>LTAKHRPSVVWLHNAECTGCTEAAIRTIKPYIDALILDTISLDYQETIMAAAGEAAEAALHQALEGKDGYYLVVEGGLPTIDGGQWGMVAGHPMIETTKKAAAKAKGIICIGTCSAYGGVQKAKPNPSQAKGVSEALGVKTINIPGCPPNPINFVGAVVHVLTKGIPDLDENGRPKLFYGELVHDNCPRLPHFEASEFAPSFDSEEAKKGFCLYELGCKGP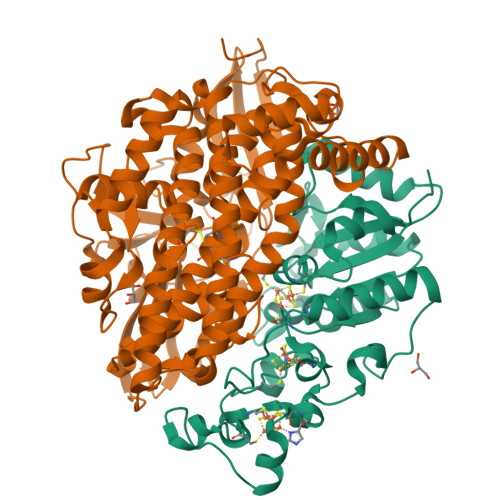VTYNNCPKVLFNQVNWPVQAGHPCLGCSEPDFWDTMTPFYEQG[3x];>[3x]MAESKPTPQSTFTGPIVVDPITRIEGHLRIMVEVENGKVKDAWSSSQLFRGLEIILKGRDPRDAQHFTQRACGICTYVHALASSRCVDDAVKVSIPANARMMRNLVMASQYLHDHLVHFYHFHALDWVDVTAALKADPNKAAKLAASIAPARPGNSAKALKAVQDKLKAFVESGQLGIFTNAYFLGGHKAYYLPPEVDLIATAHYLEALHMQVKAASAMAILGGKNPHTQFTVVGGCSNYQGLTKDPLANYLALSKEVCQFVNECYIPDLLAVAGFYKDWGGIGGTSNYLAFGEFATDDSSPEKHLATSQFPSGVITGRDLGKVDNVDLGAIYEDVKYSWYAPGGDGKHPYDGVTDPKYTKLDDKDHYSWMKAPRYKGKAMEVGPLARTFIAYAKGQPDFKKVVDMVLGKLSVPATALHSTLGRTAARGIETAIVCANMEKWIKEMADSGAKDNTLCAKWEMPEESKGVGLADAPRGALSHWIRIKGKKIDNFQLVVPSTWNLGPRGAQGDKSPVEEALIGTPIADPKRPVEILRTVHAFDPCIACGVH>[9x]MEKKITGYTTVDISQWHRKEHFEAFQSVAQCTYNQTVQLDIT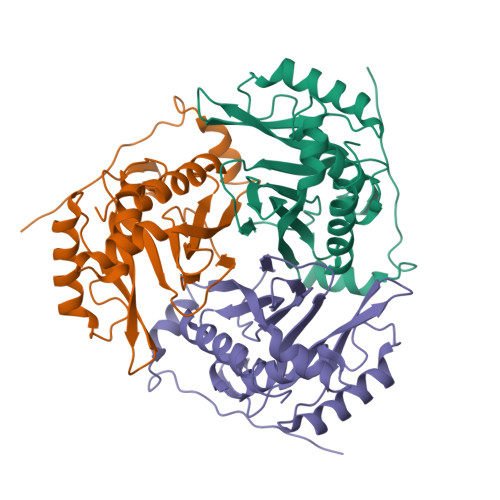AFLKTVKKNKHKFYPAFIHILARLMNAHPEFRMAMKDGELVIWDSVHPCYTVFHEQTETFSSLWSEYHDDFRQFLHIYSQDVACYGENLAYFPKGFIENMFFVSANPWVSFTSFDLNVANMDNFFAPVFTMGKYYTQGDKVLMPLAIQVHHAVCDGFHVGRMLNELQQYCDEWQGGA The sliding β-clamp polymerase processivity factor adopts a doughnut-like ring shaped structure where the DNA passes through the positively charged inner hollow of the clamp. The β-clamp itself has to be loaded onto DNA with the help of the multi-protein clamp loader complex. β-Clamps are essential for many important DNA transactions including replication and repair. It recruits various factors like DNA polymerases, ligases, and other DNA interacting/processing proteins to the ‘scene of action’. Structures of β-clamps are known from diverse sources including E. coli, T. maritima and S. pyogenes till date. These structures show that the β-clamp exists as homodimers whose protomers assemble in a head-to-tail fashion.

The structure was solved using molecular replacement (MR) techniques employing the structure of the E. coli clamp as the model for the calculations. Structurally it is similar to those of the clamps from other sources like E. coli, S. pyogenes and T. maritima. The crystal structure reveals the details of the positively charged inner ring that is involved in DNA recognition and the hydrophobic binding site that is involved in the recognition of partner proteins. The structural conservation of the Mtbβ-Clamp as seen in the crystal structures is not surprising, especially for a protein performing an important role in various pathways involving DNA. The comparative studies demonstrate that the peptide and DNA recognition region(s) in the Mtbβ-Clamp is well conserved compared to other clamps and no obvious differences could be detected in these sites to ascribe the lack of interactions of the Mtbβ-Clamp with the LigA. We find that the mycobacterial clamp also has specific affinity for DNA and exhibits about 1.8 times higher affinity for primed DNA compared to nicked and dsDNA respectively. However the affinity of both homologs for blunt dsDNA is similar with Kd 453 and 557 nM for the E. coli and M. tuberculosis clamps respectively. Mtbβ-clamp itself exhibits affinity for components of the clamp loader complex. Surprisingly we found that no direct interactions exist in vitro between MtbLigA and Mtbβ-clamp. The results therefore suggest that other as-yet-unidentified factors/mechanisms may mediate interactions between these proteins and DNA.

>[2x]VGLTDLTFRLLRESFADAVSWVAKNLPARPAVPVLSGVLLTGSDNGLTISGFDYEVSAEAQVGAEIVSPGSVLVSGRLLSDITRALPNKPVDVHVEGNRVALTCGNARFSLPTMPVEDYPTLPTLPEETGLLPAELFAEAISQVAIAAGRDDTLPMLTGIRVEILGETVVLAATDRFRLAVRELKWSASSPDIEAAVLVPAKTLAEAAKAGIGGSDVRLSLGTGPGVGKDGLLGISGNGKRSTTRLLDAEFPKFRQLLPTEHTAVATMDVAELIEAIKLVALVADRGAQVRMEFADGSVRLSAGADDVGRAEEDLVVDYAGEPLTIAFNPTYLTDGLSSLRSERVSFGFTTAGKPALLRPVSGDDRPVAGLNGNGPFPAVSTDYVYLLMPVRLPG> MRGSHHHHHHGSMAERKGTAKVDFLKKIEKEIQQKWDTERVFEVNASNLEKQTSKGKYFVTFPYPYMNGRLHLGHTFSLSKCEFAVGYQRLKGKCCLFPFGLHCTGMPIKACADKLKREIELYGCPPDFPDEEEEEEETSVKTEDIIIKDKAKGKKSKAAAKAGSSKYQWGIMKSLGLSDEEIVKFSEAEHWLDYFPPLAIQDLKRMGLKVDWRRSFITTDVNPYYDSFVRWQFLTLRERNKIKFGKRYTIYSPKDGQPCMDHDRQTGEGVGPQEYTLLKLKVLEPYPSKLSGLKGKNIFLVAATLRPETMFGQTNCWVRPDMKYIGFETVNGDIFICTQKAARNMSYQGFTKDNGVVPVVKELMGEEILGA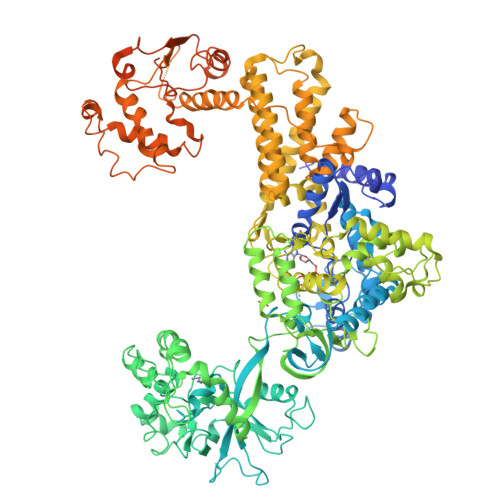SLSAPLTSYKVIYVLPMLTIKEDKGTGVVTSVPSDSPDDIAALRDLKKKQALRAKYGIRDDMVLPFEPVPVIEIPGFGNLSAVTICDELKIQSQNDREKLAEAKEKIYLKGFYEGIMLVDGFKGQKVQDVKKTIQKKMIDAGDALIYMEPEKQVMSRSSDECVVALCDQWYLDYGEENWKKQTSQCLKNLETFCEETRRNFEATLGWLQEHACSRTYGLGTHLPWDEQWLIESLSDSTIYMAFYTVAHLLQGGNLHGQAESPLGIRPQQMTKEVWDYVFFKEAPFPKTQIAKEKLDQLKQEFEFWYPVDLRVSGKDLVPNHLSYYLYNHVAMWPEQSDKWPTAVRANGHLLLNSEKMSKSTGNFLTLTQAIDKFSADGMRLALADAGDTVEDANFVEAMADAGILRLYTWVEWVKEMVANWDSLRSGPASTFNDRVFASELNAGIIKTDQNYEKMMFKEALKTGFFEFQAAKDKYRELAVEGMHRELVFRFIEVQTLLLAPFCPHLCEHIWTLLGKPDSIMNASWPVAGPVNEVLIHSSQYLMEVTHDLRLRLKNYMMPAKGKKTDKQPLQKPSHCTIYVAKNYPPWQHTTLSVLRKHFEANNGKLPDNKVIASELGSMPELKKYMKKVMPFVAMIKENLEKMGPRILDLQLEFDEKAVLMENIVYLTNSLELEHIEVKFASEAEDKIREDCCPGKPLNVFRIEPGVSVSLVNPQPSNGHFSTKIEIRQGDNCDSIIRRLMKMNRGIKDLSKVKLMRFDDPLLGPRRVPVLGKEYTEKTPISEHAVFNVDLMSKKIHLTENGIRVDIGDTIIYLVH> DEVTSTT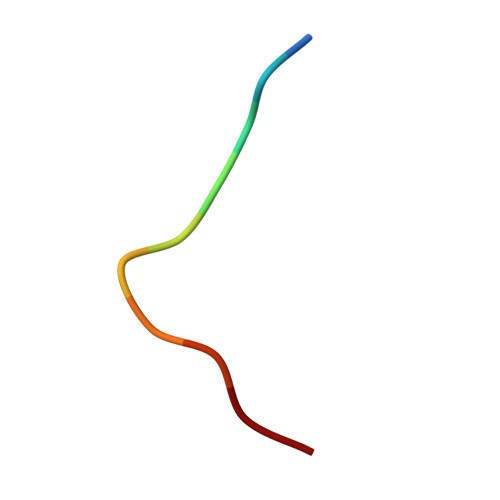SSS>[2x]GPLGSMGSVLSSGQPTEEQLKMALQKAQQLVNSNPLVVFSKTYAGYCSRVKKLFDQLGARYQTIELDQESDGDAIQAALLQ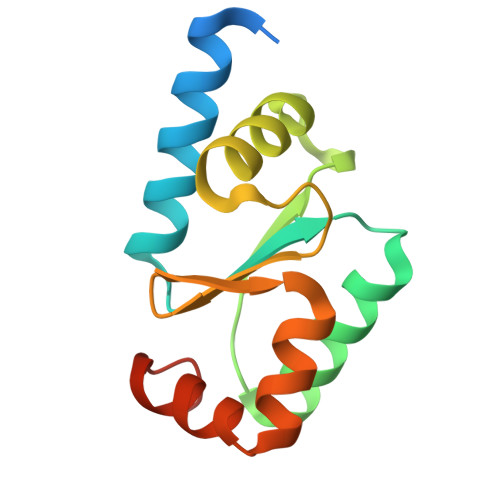WTGQRTVPNVFIGGKHIGGCDSVMEKHRDGKLVPMLTECGAIAIESTA>MPEGPELHLASQFVNEACRALVFGGCVEKSSVSRNPEVPFESSAYRISASARGKELRLILSPLPGAQPQQEPLALVFRFGMSGSFQLVPREELPRHAHLRFYTAPPGPRLALCFVDIRRFGRWDLGGKWQPGRGPCVLQEYQQFRENVLRNLADKAFDRPICEALLDQRFFNGIGNYLRAEILYRLKIPPFEKARSVLEALQQHRPSPELTLSQKIRTKLQNPDLLELCHSVPKEVVQLGGRGRGSESGEEDFAAFRAWLRCY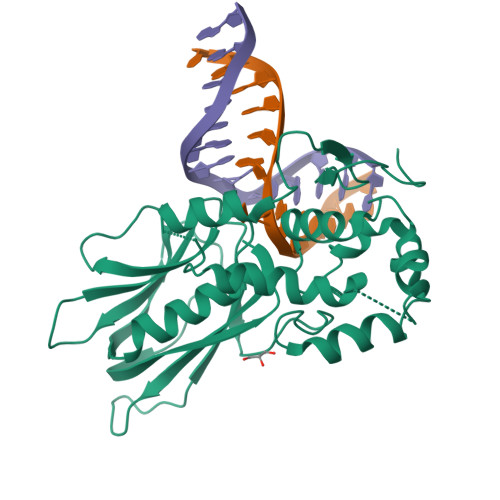GMPGMSSLQDRHGRTIWFQGDPGPLAPKGRKS[3x]>MLAILYDRIRPDERMLFERAEALGLPYKKVYVPALPMVLGERPKELEGVTVALERCVSQSRGLAAARYLTALGIPVVNRPEVIEACGDKWATSVALAKAGLPQPKTALATDREEALRLMEAFGYPVVLKPVIGSWGRLLAXXXXXXXXXXXXXXKEVLGGFQHQLFYIQEYVEKPGRDIRVFVVGERAIAAIYRRSAHWITNTARGGQAENCPLTEE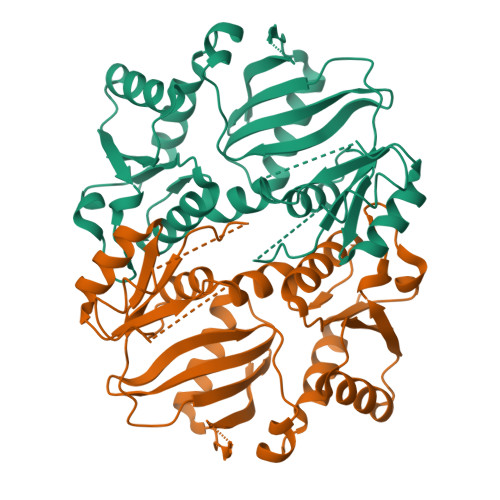VARLSVKAAEAVGGGVVAVDLFESERGLLVNEVNHTMEFKNSVHTTGVDIPGEILKYAWSLAS[2x]>EIPLKYGATNEGKRQDPAMQKFRDNRLGAFIHWGLYAIPGGEWNGKVYGGAAEWLKSWAKVPADEWLKLMDQWNPTKFDAKKWAKMAKEMGTKYVKITTKHHEGFCLWPSKYTKYTVANTPYKRDILGELVKAYNDEGIDVHFYFSVMDWSNPDYRYDIKSKEDSIAFSRFLEFTDNQLKELATRYPTVKDFWFDGTWDASVKKNGWWTAHAEQMLKELVPGVAINSRLRADDKGKRHFDSNGRLMGDYESGYERRLPDPVKDLKVTQWDWEACMTIPENQWGYHKDWSLSYVKTPIEVIDRIVHAVSMGGNMVVNFGPQADGDFRPEEKAMATAIGKWMNRYGKAVYACDYAGFEKQDWGYYTRGKNDEVYMVVFNQPYSERLIVKTPKGITVEKATLLTTGEDITVVETTRNEYNVSVPKKNPGEPYVIQLKVRAAKGTKSIYRDALT[3x];> EIPLKYGATNEGKRQDPAMQKFRDNRLGAFIHWGLYAIPGGEWNGKVYGGAAEWLKSWAKVPADEWLKLMDQWNPTKFDAKKWAKMAKEMGTKYVKITTKHHEGFCLWPSKYTKYTVANTPYKRDILGELVKAYNDEGIDVHFYFSVMDWSNPDYRYDIKSKEDSIAFSRFLEFTDNQLKELATRYPTVKDFWFDGTWDASVKKNGWWTAHAEQMLKELVPGVAINSRLRADDKGKRHFDSNGRLMGDYESGYERRLPDPVKDLKVTQWDWEACMTIPENQWGYHKDWSLSYVKTPIEVIDRIVHAVSMGGNMVVNFGPQADGDFRPEEKAMATAIGKWMNRYGKAVYACDYAGFEKQDWGYYTRGKNDEVYMVVFNQPYSERLIVKTPKGITVEKATLLTTGEDITV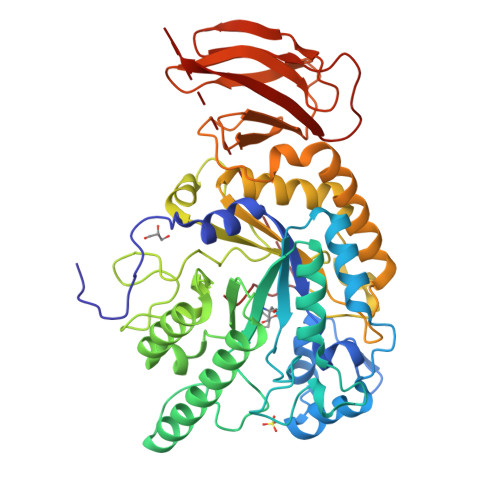VETTRNEYNVSVPKKNPGEPYVIQLKVRAAKGTKSLYRDALT>MASMTGGQQMGAPITAYAQQTRGLLGCIITSLTGRDKNQVEGEVQIVSTATQTFLATCINGVCWTVYHGAGTRTIASPKGPVIQMYTNVDQDLVGWPAPQGSRSLTPCTCGSSDLYLVTRHADVIPVRRRGDSRGSLLSPRPISYLKGS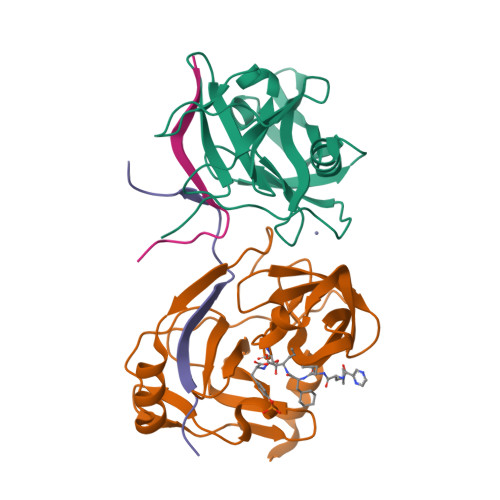SGGPLLCPAGHAVGLFRAAVCTRGVTKAVDFIPVENLETTMRSGSHHHHHH[2x];>KGSVVIVGRIVLSGKPAIIPKK[2x]> MERYENLFAQLNDRREGAFVPFVTLGDPG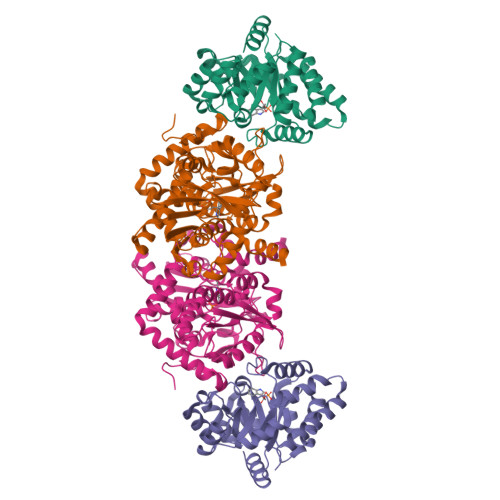IEQSLKIIDTLIDAGADALELGVPFSDPLADGPTIQNANLRAFAAGVTPAQCFEMLALIREKHPTIPIGLLMYANLVFNNGIDAFYARCEQVGVDSVLVADVPVEESAPFRQAALRHNIAPIFICPPNADDDLLRQVASYGRGYTYLLSRSGVTGAENRGALPLHHLIEKLKEYHAAPALQGFGISSPEQVSAAVRAGAAGAISGSAIVKIIEKNLASPKQMLAELRSFVSAMKAASRA;> TTLLNPYFGEFGGMYVPQILMPALNQLEEAFVSAQKDPEFQAQFADLLKNYAGRPTALTKCQNITAGTRTTLYLKREDLLHGGAHKTNQVLGQALLAKRMGKSEIIAETGAGQHGVASALASALLGLKCRIYMGAKDVERQSPNVFRMRLMGAEVIPVHSGSATLKDACNEALADWSGSYETAHYMLGTAAGPHPYPTIVREFQRMIGEETKAQILDKEGRLPDAVIACVGGGSNAIGMFADFINDTSVGLIGVEPGGHGIETGEHGAPLKHGRVGIYFGMKAPMMQTADGQIEESYSISAGLDFPSVGPQHAYLNSIGRADYVSITDDEALEAFKTLCRHEGIIPALESSHALAHALKMMREQPEKEQLLVVNLSGRGDKDIFTVHDILKARGEI> GPGSEFELRRQASNYQLTLTNTRATVNILMERLKKSDADVEQYRAELESVQLAKGALE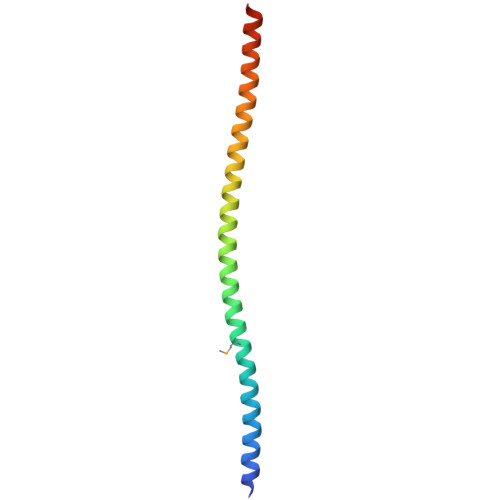QSYLVLQADAEQLRQQLTESQDALNALRSSSQTLQSE[(2R,3S,4R,5R)-5-(6-AMINOPURIN-9-YL)-3,4-DIHYDROXY-OXOLAN-2-YL]METHYL [[(2R,3R)-2,3-DIHYDROXY-4-OXO-PENTOXY]-OXIDO-PHOSPHORYL] PHOSPHATE | C15 H21 N5 O13 P2 | 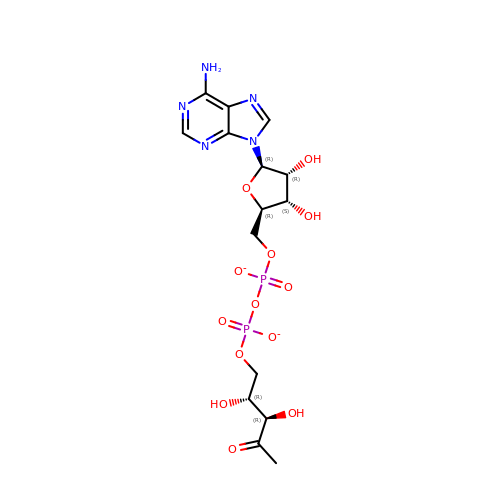IZTPERUWNZCNNH-GHVQHMAVSA-L4,4,4-trifluoro-1-(4-nitrophenyl)butane-1,3-dione | C10 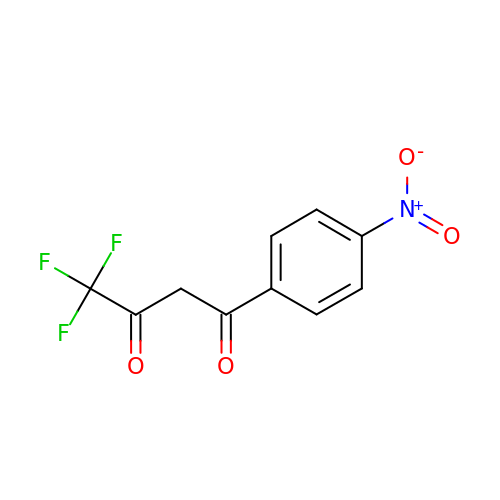H6 F3 N O4 | CDSAMNVLRSHLPN-UHFFFAOYSA-N>LPRPIRNLEVKFTKIFINNEWHESKSGKKFATCNPSTREQICEVEEGDKPDVDKAVEAAQVAFQRGSPWRRLDALSRGRLLHQLADLVERDRATLAALETMDTGKPFLHAFFIDLEGCIRTLRYFAGWADKIQGKTIPTDDNVVCFTRHEPIGVCGAITPWNFPLLMLVWKLAPALCCGNTMVLKPAEQTPLTALYLGSLIKEAGFPPGVVNIVPGFGPTVGAAISSHPQINKIAFTGSTEVGKLVKEAASRSNLKRVTLELGGKNPCIVCADADLDLAVECAHQGVFFNQGQCCTAASRVFVEEQVYSEFVRRSVEYAKKRPVGDPFDVKTEQGPQIDQKQFDKILELIESGKKEGAKLECGGSAMEDKGLFIKPTVFSEVTDNMRIAKEEIFGPVQPILKFKSIEEVIKRANSTDYGLTAAVFTKNLDKALKLASALESGTVWINCYNALYAQAPFGGFKMSGNGRELGEYALAEYTEVKTVTIKLG[2x]

The human aldehyde dehydrogenase (ALDH) superfamily comprises 19 enzyme isoforms catalyzing the NAD(P)-dependent irreversible oxidation of aldehydes to their corresponding carboxylic acids. Cytosolic ALDH1A enzymes, and specifically the ALDH1A3 isoform, are good markers of cancer stem cells and have been implicated in carcinogenesis, chemoresistance and relapse. As previously observed in other members of the enzyme superfamily, each ALDH1A3 subunit is composed of three structural domains: a catalytic domain, a cofactor-binding domain and an oligomerization domain. At the intersection of the substrate- and cofactor-binding pockets sits a strictly conserved cysteine residue (Cys302, ALDH2 numbering), which is essential for catalysis, acting as the active-site nucleophile.

The ALDH1A3-ATP structure at 1.78-Å resolution contains one ATP molecule in each subunit. The ATP molecule in monomers A and B is located in the adenosine-binding moiety of the cofactor-binding pocket and is accommodated via direct hydrogen bonding with Thr178, Trp180, Lys204, Glu207, and Ser258, and via hydrophobic interactions with ten additional residues (right). The α- and β-phosphate groups of ATP have identical interactions to those of the NAD+ pyrophosphate, including four water molecules, while the γ-phosphate group is not showing any specific interaction. As anticipated, the average B-factor increased from α- to γ-phosphate groups of ATP (66–72 Å2), being highest for the latter, indicating more flexibility at this end of the ATP molecule. The ALDH1A3-ATP structure also contains two PEG molecules (PEG1 and PEG2) inside the substrate-binding pocket in monomers A and B. However, in this case, the PEG1 molecule is covalently bound to Cy314 in both subunits with a distance between Sγ-Cys314 and C1-PEG1 atoms of 1.82 and 1.83 Å for monomers A and B, respectively, which is a typical distance for a covalent C − S bond. The O1-PEG1 atom is hydrogen bonded to the N-Cys314 and Nδ2-Asn181 atoms in both monomers and occupies the position of the water molecule near Cys314 in the ALDH1A3-NAD+ structure. The genuine interest of the ALDH1A3-ATP structure is that it can be interpreted as a true thioacyl-enzyme intermediate in the ALDH catalytic mechanism, which is trapped in a dead enzyme lacking an active cofactor. The role of Asn181 in stabilizing the reaction intermediate through hydrogen bonding with the O atom of the carbonyl substrate, as suggested by our results, is consistent with similar bonds observed in other ALDH ternary complexes. At physiological concentrations, ATP inhibits the dehydrogenase activity of ALDH1A3 and other isoforms, with a Ki value of 0.48 mM for ALDH1A3, showing a mixed inhibition type against NAD+.Tc toxins consist of three components: TcA, TcB, and TcC. The ~1.4 MDa TcA is a homo-pentameric bell-shaped molecule that mediates target cell association, membrane penetration, and toxin translocation. TcA is made up of a central, pre-formed channel that is enclosed by an outer shell composed of a structurally conserved α-helical domain decorated with variable receptor-binding domains (RBDs). Cryo-EM structures of Mm-TcdA4 and Xn-XptA1 in complex with heparin reveal that the glycan interacts with different parts of the shell domain, including receptor-binding domains.

To address whether heparins/HS bind to a different region in other TcAs, we decided to determine the structure of a TcA from another organism in complex with heparin/HS. We chose Xn-XptA1, because it also shows a strong binding signal to porcine intestinal mucosa heparin. Expectedly, the obtained cryo-EM structure at 3.7 Å resolution is very similar to the structure of Xn-XptA1 without heparin, but clear densities corresponding to heparin/HS are present. However, their position differs from that in the Mm-TcdA4–heparin complex. Instead of interacting with the upper region of the shell, they are located in a gap between the neuraminidase-like domain, RBD B and RBD D. This binding pocket is not directly connected to the α-helical shell and is predominantly formed by polar and charged residues. In particular, a docked heparin oligosaccharide interacts with N1090, N1092, H1121, D1582, and S1584 of the neuraminidase-like domain, Y1548 and S1580 of RBD B and W1663, K1665, N1674, R1677, Q1678, and P1679 of RBD D. Since the RBDs of Tc toxins are not conserved, this binding pocket is not conserved as well. In the case of Xn-XptA1, the heparin/HS binding site is closer to the membrane (ca. 4 nm) and is located in a cleft between two RBDs and the neuraminidase-like domain. Taken together, our results show that the heparin/HS binding site is not conserved in different TcAs, although binding itself is.

>MIKVNELLDKINRKRSGDTLLLTNISFMSFSEFRHRTSGTLTWRETDFLYQQAHQESKQNKLEELRILSRANPQLANITNLNITPSTLNNSYNSWFYGRAHRFVKPGSIASIFSPAAYLTELYREAKDFHPDNSQYHLNKRRPDIASLALTQNNMDEEISTLSLSNELLLHNIQTLEKTDYNGVMKMLSTYRQTGMTPYHLPYESARQAILLQDKNLTAFSRNTDVAELMDPTSLLAIKTDISPELYQILVEEITPENSTELMKKNFGTDDVLIFKSYASLARYYDLSYDELSLFVNLSFGKKNTNQQYKNEQLITLVNDGNDTATARLIKRTRKDFYDSHLNYAELIPIKENEYKYNFSVKKTEPDHLDFRLQNGDKEYIYQDKNFVPIANTHYSIPIKLTTEQITNGITLRLWRVKPNPSDAINANAHFKMMEFPGDIFLLKLNKAIRLYKATGISPEDIWQVIESIYDDLTIDSNVLGKLFYVQYYMQHYNISVSDALVLCHSDISQYSTKQQPSHFTMLFNTPLLNGQEFSADNTKLDLTPGESKNHFYLGIMKRAFRVNDTELYTLWKLANGGTNPEFMCSIENLSLLYRVRLLADIHHLTVNELSMLLSVSPYVNTKIALFSDTALTQLISFLFQCTQWLTTQKWSVSDVFLMTTDNYSTVLTPDIENLITTLSNGLSTLSLGDDELIRAAAPLIAASIQMDSAKTAETILLWINQIKPQGLTFDDFMIIAANRDRSENETSNMVAFCQVLGQLSLIVRNIGLSENELTLLVTKPEKFQSETTALQHDLPTLQALTRFHAVIMRCGSYATEILTALELGALTAEQLAVALKFDAQVVTQALQQTDLGVNTFTNWRTIDVTLQWLDVAATLGITPDGVAALIKLKYVGEPETPMPTFDDWQAASTLLQAGLNSQQSDQLQAWLDEATTTAASAYYIKNGAPQQIKSRDELYSYLLIDNQVSAQVKTTRVAEAIASIQLYVNRALNNVEGKVSKPVKTRQFFCDWETYNRRYSTWAGVSELAYYPENYIDPTIRIGQTGMMNNLLQQLSQSQLNIDTVEDSFKNYLTAFEDVANLQVISGYHDSINVNEGLTYLIGYSQTEPRIYYWRNVDHQKCQHGQFAANAWGEWKKIEIPINVWQENIRPVIYKSRLYLLWLEQKELKNESEDGKIDITDYILKLSHIRYDGSWSSPFNFNVTDKIENLINKKASIGMYCSSDYEKDVIIVYFHEKKDNYSFNSLPAREGMTINPDMTLSILTENDLDAIVKSTLSELDTRTEYKVNNQFATDYLAEYKESITTKNKLASFTGNIFDLSYISPGNGHINLTFNPSMEINFSKGNIYNDEVKYLLSMVEDETVILFDYDRHDEMLGKEEEVFHYGTLDFIISIDLKNAEYFRVLMHLRTKEKIPRKSEIGVGINYDYESNDAEFKLDTNIVLDWKDNTGVWHTICESFTNDVSIINNMGNIAALFLREDPCVYLCSIATDIKIASSMIEQIQDKNISFLLKNGSDILVELNAEDHVASKPSHESDPMVYDFNQVKVDIEGYDIPLVSEFIIKQPDGGYNDIVIESPIHIKLKSKDTSNVISLHKMPSGTQYMQIGPYRTRLNTLFSRKLAERANIGIDNVLSMETQNLPEPQLGEGFYATFKLPPYNKEEHGDERWFKIHIGNIDGNSARQPYYEGMLSDIETTVTLFVPYAKGYYIREGVRLGVGYKKIIYDKSWESAFFYFDETKNQFIFINDADHDSGMTQQGIVKNIKKYKGFIHVVVMKNNTEPMDFNGANAIYFWELFYYTPMMVFQRLLQEQNFTESTRWLRYIWNPAGYSVQGEMQDYYWNVRPLEEDTSWNANPLDSVDPDAVAQHDPMHYKVATFMKMLDLLITRGDSAYRQLERDTLNEAKMWYVQALTLLGDEPYFSLDNDWSEPRLEEAASQTMRHHYQHKMLQLRQRAALPTKRTANSLTALFLPQINKKLQGYWQTLTQRLYNLRHNLTIDGQPLSLSLYATPADPSMLLSAAITASQGGGDLPHAVMPMYRFPVILENAKWGVSQLIQFGNTLLSITERQDAEALAEILQTQGSELALQSIKMQDKVMAEIDADKLALQESRHGAQSRFDSFNTLYDEDVNAGEKQAMDLYLSSSVLSTSGTALHMAAAAADLVPNIYGFAVGGSRFGALFNASAIGIEISASATRIAADKISQSEIYRRRRQEWEIQRNNAEAEIKQIDAQLATLAVRREAAVLQKNYLETQQAQTQAQLAFLQSKFSNAALYNWLRGRLSAIYYQFYDLAVSLCLMAEQTYQYELNNAAAHFIKPGAWHGTYAGLLAGETLMLNLAQMEKSYLEKDERALEVTRTVSLAEVYAGLTENSFILKDKVTELVNAGEGSAGTTLNGLNVEGTQLQASLKLSDLNIATDYPDGLGNTRRIKQISVTLPALLGPYQDVRAILSYGGSTMMPRGCKAIAISHGMNDSGQFQMDFNDAKYLPFEGLPVADTGTLTLSFPGISGKQKSLLLSLSDIILHIRYTIRS[5x]BROMAMPHENICOL | C11 H12 Br2 N2 O5 | 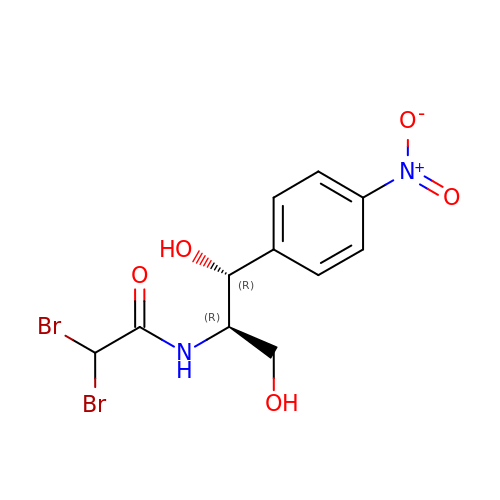UWOHGNMWBGIRAQ-RKDXNWHRSA-N> DGMTAAQARQMESLNRGLVAVKTGNGVFVSWRLLGTEPSSVSFNVYRNGKKLNGSPITSSTNYQDAGGDLNAVYQVRAVLNGRE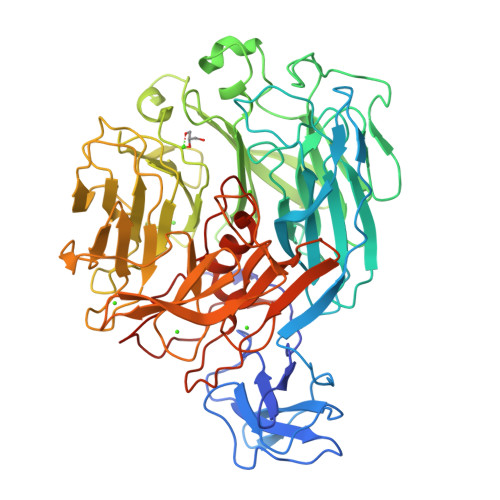QAPSESVGVLNKQYKSVPLQKPAGGKTPDGVSYTYSANDASVGDLDGDGQYEIILKWDPSNSKDNSQDGYTGDVLIDAYKLDGTMMWRINLGKNIRAGAHYTQFLVYDFDGDGKAEIAMKTADGTKDGKGKVIGNANADYRNAQGRILSGPEYLTVFKGDTGAELTTVNYEPARGNVADWGDSYGNRVDRFLAGVAYLDGERPSFVMARGYYTRTVLVAYNFRGGKLTKLWTFDSDAPGNGAYAGQGNHSLSVADVDGDGKDEIIYGAMAVDHDGKGLYSTGWGHGDAMHTGNLDPSRPGLEVFQVHENSNSPYGLSFRDAKTGKIIWGVHAGKDVGRGMAADIDPRYEGAEVWANGSLYTAKGVKIGNTLPSSTNFGIWWDGDLQRELLDSNRIDKWDYQNSRTVNLLTASGASANNGTKATPSLQADILGDWREEVVWRAEDSSELRIYTTTDVTEHRMYTLMHDAVYRLGIAWQNVGYNQPPHTGFYLGEGMQTPEKPNIYTRHHHHHH The viral genome is encapsidated in a sheath of oligomerized copies of the nucleoprotein N, forming a ribonucleoprotein complex termed nucleocapsid. The nucleocapsid is the template for transcription and replication by L, which is also dependent on the obligate polymerase cofactor, the phosphoprotein P, together forming the active L/P holoenzyme. In oligomerized and RNA-bound N (N-RNA) the nucleic acid is threaded along an extended groove in between the NTDs and CTDs of laterally connected N protomers. An important function of the C-terminal domain of P in nsNSVs is to bind to assembled N-RNA, forming an N-RNA/P complex.

We incubated N-RNA preparations with a ~ 100-fold molar excess of synthetic peptide covering the 9 last residues of PCT (N-EDDIYQLIM-C). In the reconstructions, additional density was visible at the periphery of the NTD of N. To facilitate easier model building and to obtain improved maps, we carried out symmetry expansion and local refinement of a dimer of N-RNA/P as before with N-RNA. The final resolution was at 2.9 Å and comparison of the N-RNA and N-RNA/P dimer maps revealed a density of sufficient quality to allow refinement of a model of the bound PCT. The locally refined cryo-EM map resolved the residues 288 to 294 of the PCT bound to N-RNA. PCT is wedged in between a helix of N (N residues 121-141, helix αI2, RSV numbering) on one side and an extended loop of a beta-hairpin of N (NβHL, N residues 99-112) on the other, burying a total area of ~1100 Å2 upon complex formation. We observed a noticeable increase in ordered density of NβHL upon P-binding, compared to the apo form (black arrow). We observe that the P peptide wraps around a central arginine at position R132 belonging to helix αI2.P hooks onto this arginine by packing the hydrophobic surfaces of PCT side-chains P-M294, P-L292, P-I289, and P-Y290 against the aliphatic chain of R132, thereby completely surrounding it. R132 is additionally stabilized and kept in position through a polar contact with D128. The C-terminal methionine of P (P-M294) inserts into a hydrophobic cavity on N formed by L46 and M135. Moreover, the face of the aromatic ring of P-Y290 packs against three hydrophobic residues located within NβHL: L100, I103, and L111.

>[2x]MSLQGIHLSDLSYKHAILKESQYTIKRDVGTTTAVTPSSLQQEITLLCGEILYAKHADYKYAAEIGIQYISTALGSERVQQILRNSGSEVQVVLTRTYSLGKIKNNKGEDLQMLDIHGVEKSWVEEIDKEARKTMATLLKESSGNIPQNQRPSAPDTPIILLCVGALIFTKLASTIEVGLETTVRRANRVLSDALKRYPRMDIPKIARSFYDLFEQKVYHRSLFIEYGKALGSSSTGSKAESLFVNIFMQAYGAGQTMLRWGVIARSSNNIMLGHVSVQAELKQVTEVYDLVREMGPESGLLHLRQSPKAGLLSLANCPNFASVVLGNASGLGIIGMYRGRVPNTELFSAAESYAKSLKESNKINFSSLGLTDEEKEAAEHFLNVSDDSQNDYE;>[2x]DIYQLIM(2S)-2-{4'-[(6-aminopyridin-3-yl)sulfonyl]biphenyl-4-yl}-1,1,1-trifluoropropan-2-ol 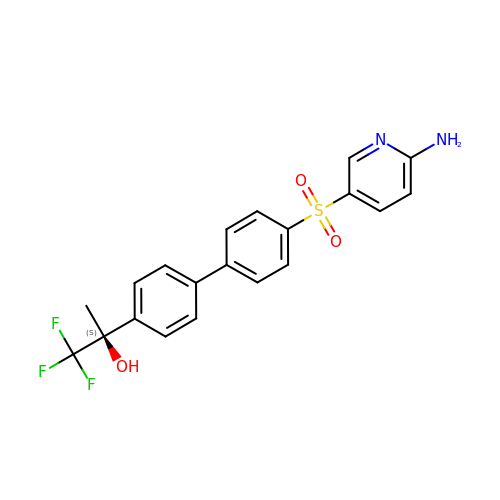| C20 H17 F3 N2 O3 S | XOWBHNIRCZERRH-IBGZPJMESA-N> WLDFSDSASWKNLDQRGGLKVGTTFTKEISPGYVVTLTVKELKPFNSTEIYKKRVAGTATEGTYDPDAENGFLTSAPYYGKTPPPSVTGAAQNEWTTIRDQGFNTQKRKTQLVYPMNSTNWGVKFDIEATYLGKR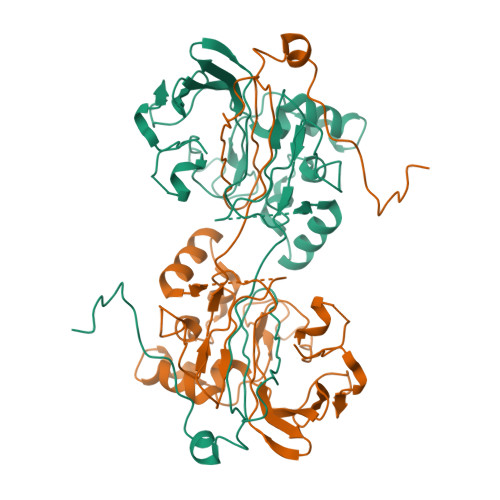VAPTVVMADGEDANPGEFAIFTTNGTGWEYMGEWKMKSPAKEAYNVITKKMLDDEDVKRRGLLILKDKSVDWYKYLSPDTVTGGLGSQVFGPNRSNERTVPVVMTRGASEVGFYVASSGQQAMMMGFLVVAVSDAPESYGEAFHTISTRDSVTNDPINQPYLGTTPADIDVESSNDWVLDDKK> SLSAAEADLAGKSWAPVFANKNANGDAFLVALFEKFPDSANFFADFKGKSVADIKASPKLRDHSSTIFTRLNEFVNNAANAGKMSAMLSQFAKEHVGFGVGSAQFENVRSMFPGFVASVAAPPAGADAAWTKLFGL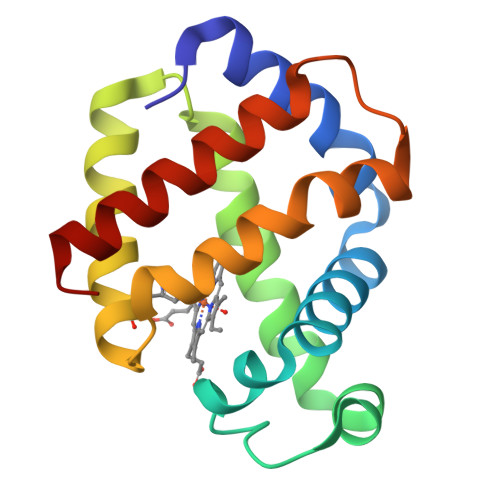IIDALKAAGK> GAMDHVEFGLTYSQLMTLKDAMLQLDPNAKTWMDIEGRPEDPVEIALYQPSSGCYIHFFREPTDLKQFKQDAKYSHGIDVTDLFATQPGLTSAVIDALPRNMVITCQGSDDIRKLLESQGRKDIKLIDIALSKTDSRKYENAVWDQYKDLCHMHTGVVVEKKKRGGKEEITPHCALMDCIMFDAAVSGGLNTSVLRAVLPRDMVFRTSTPRVVL

Lassa virus (LASV) nucleoprotein (NP) is the only known 3′-5′ exoribonuclease that can suppress type I interferon (IFN) production possibly by degrading immune-stimulatory RNAs. NP is a multifunctional protein involved in viral genomic RNA encapsidation, viral RNA synthesis, and immune evasion. Our structural, biochemical, and cell-based analyses have demonstrated that NP encodes a functional 3′-5′ exoribonuclease of the DEDDH family at its C terminus and that this RNase activity plays a strikingly important role in IFN suppression. We therefore propose a novel immune evasion mechanism in which NP suppresses the IFN induction by selectively degrading these immune-stimulatory RNAs.

We obtained crystals of NP-C in the presence of an 8-bp dsRNA oligo (5′-GGGCGCCC-3′/3′-CCCGCGGG-5′) with either 5′-OH or 5′-triphosphate (5′-ppp), with the 5′-ppp dsRNA complex diffracted to a much higher resolution (1.68 Å). These crystals belong to a space group of P41212 with unit cell dimensions of a = 46.74 Å, b = 46.74 Å, c = 217.31 Å, and α = β = γ = 90°. Single asymmetric unit cells contain one NP-C monomer bound to an RNA substrate. The electrostatic surface potential map shows that the dsRNA-binding surface, with a surface area of 606 Å2, is highly positively charged. Electron density of the RNA substrate clearly showed the presence of 4 bp (5′-GGGC-3′/3′-CCCG-5′) in the catalytic cavity. For convenience, the 8-bp RNA is numbered as 5′-G1G2G3C4G5C6C7C8–3′. This was because a catalytically active NP-C domain was used in the co-crystallization process and was predicted to have removed the last 4 nucleotides from the 3′ end of the cleaving strand, resulting in an intermediate dsRNA product with a 5′ protruding end of the complementary strand (5′-GGGC-3′/3′-CCCGCGGG-5′). The 4 nucleotides 5′-GGGC-3′ of the cleaving strand were almost completely buried in the catalytic cavity. In particular, the 3′-end ribonucleotide C at position 4 of the cleaving strand was coordinately anchored by several residues: Arg-492 through a water molecule forming a hydrogen bridge with the phosphate group, and Arg-426 and Glu-391 through their side chains forming a hydrogen bond with the 2′- and 3′-oxygen of the ribose of the cytosine ribonucleoside, respectively. Remarkably, the 3′-end ribonucleotide C of the cleaving strand was positioned precisely in the deep pocket of the catalytic site, with the terminal bond of the ribonucleotide completely exposed to the catalytic residues for hydrolysis.>[8x]MGHHHHHHHHEFIPSNTDYPGPHHFEVTFQQSSTAKSATWTYSPLLKKLYCQIAKTCPIQIKVSTPPPPGTAIRAMPVYKKAEHVTDVVKRCPNHE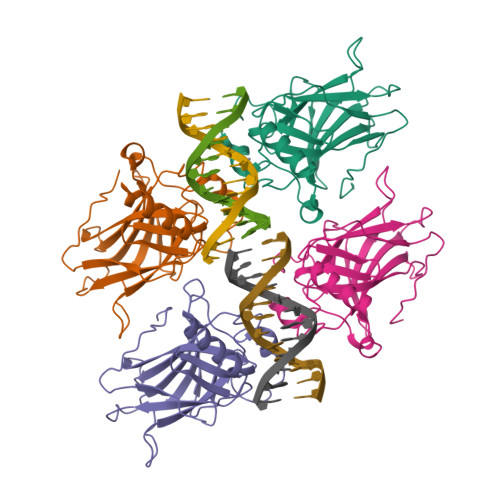LGRDFNEGQSAPASHLIRVEGNNLSQYVDDPVTGRQSVVVPYEPPQVGTEFTTILYNFMCNSSCVGGMNRRPILIIITLEMRDGQVLGRRSFEGRICACPGRDRKADEDHYREQ>MLEDLIGKAYLESAEDRRRGDRSEEVEAIRKYIRSARRTVVPNWNAEKVDAINDVLRSFNLREAEHLQFNTNWADLTRMPAVTKALMALDISGADLVIARGRLGVPGSGSLLVIMDSRGRLLSAAMSPPHV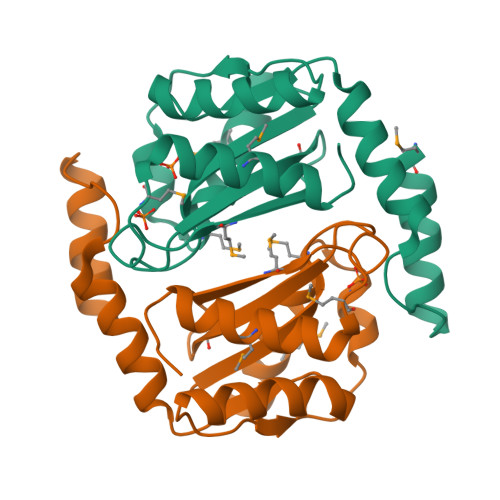IHSMEVREAVRSEMTHALERIGFKR[2x]>[2x]MPPYTVVYFPVRGRCAALRMLLADQGQSWKEEVVTVETWQEGSLKASCLYGQLPKFQDGDLTLYQSNTILRHLGRTLGLYGKDQQEAALVDMVNDGVEDLRCKYISLIYTNYEAGKDDYVKALPGQLKPFETLLSQNQGGKTFIVGDQISFADYNLLDLLLIHEVLAPGCLDAFPLLSAYVGRLSARPKLKAFLASPEYVNLPINGNGKQ

Glutathione S-transferases (GST) are involved in the metabolism of PEITC by catalyzing its conjugation with glutathione (GSH). As phase II detoxification enzymes, cytosolic GSTs exist and function as stable homo- or heterodimers. The dimer is required to maintain the functional conformations at the GSH-binding site and xenobiotic substrate-binding site in each subunit. Here, we report the crystal structures of hGSTP1 and hGSTA1 in complex with GS-PEITC (hGSTP1:GS-PEITC and hGSTA1:GS-PEITC, respectively).

We determined the crystal structures of the hGSTA1:GS-PEITC and hGSTP1:GS-PEITC complexes at 1.93- and 1.95-Å resolution, respectively. The structures show that the orientation of the phenethyl moiety of the conjugate was significantly different in the two GST enzymes. In the hGSTP1:GS-PEITC structure, however, it points toward the solvent channel, stacking with the hydrophobic side chains of Ile104 and Tyr108. The binding pocket for the phenethyl moiety of GS-PEITC in hGSTP1 can accommodate more diverse and bigger ligands than that in hGSTA1. Unlike hGSTA1 that contains only one cysteine residue, hGSTP1 contains four (Cys14, Cys47, Cys101, and Cys169). High-resolution MS showed that the modification of these cysteine side chains by PEITC resulted in multiple species of modified hGSTP1 proteins, including 1-, 2-, 3, and 4-Cys adducts. Therefore, unmodified and many species of modified hGSTP1 proteins were present in the crystal lattice at the same time, none of which was as abundant as could be revealed by observable electron density. As expected, the hGSTP1:GS-PEITC structure did not show any modified cysteine side chain. Among the four cysteine pairs in the hGSTP1 dimer, only the Cys101 pair is located in the solvent channel at the subunit interface. Because the solvent channel becomes much narrower near the bottom, there is not enough room for the covalent modifications of both Cys101 side chains at the same time.>[3x]MGSSHHHHHHSSGRENLYFQGM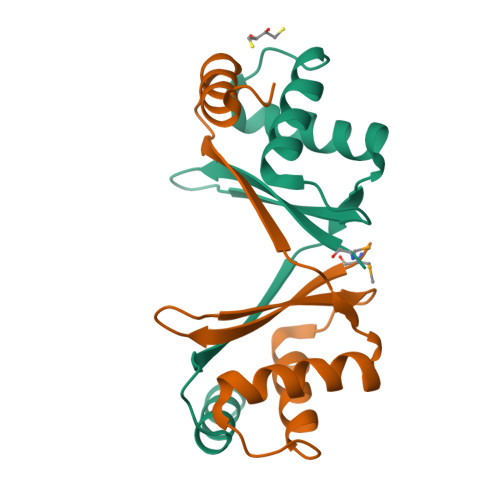RGDDMHIYELVSRDRTHPVRIYLLHSEYWTEDEFYNLLLEAFQRSSASDWHLQILEVSKYLVTAHGFVEAGGLQEIGFPGELSKTEVRRRINAFLGKDRSDGS>MPFEIVFEGAKEFAQLIDTASKLIDEAAFKVTEDGISMRAMDPSRVVLIDLNLPSSIFSKYEVVEPETIGVNLDHLKKILKRGKAKDTLILKKGEENFLEITIQGTATRTFRVPLIDVEEMEVDLPELPFTAKVVVLGEVLKAAVKAASLVSDSIKFIARE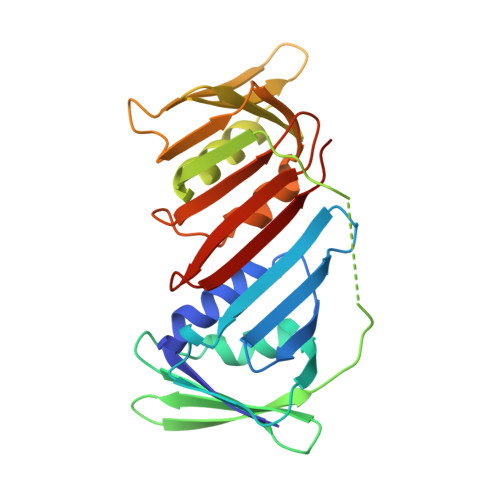NEFIMKAEGETQEVEIKLTLEDEGLLDIEVQEETKSAYGVSYLSDMVKGLGKADEVTIKFGNEMPMQMEYYIRDEGRLTFLLAPRVEE[2x]>[2x]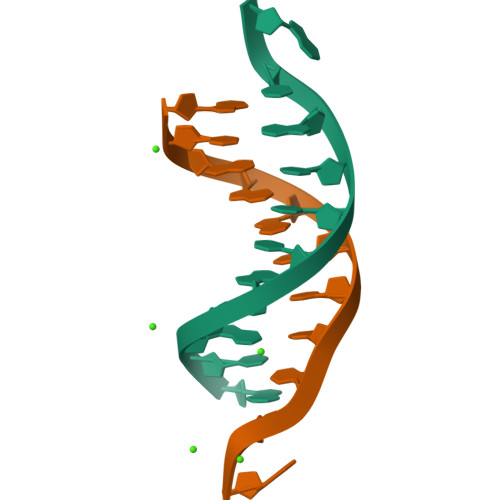GCGAATTCGCG>SNAGGSSPITGLVYDQRMMLHHNMWDSHHPELPQRISRIFSRHEELRLLSRCHRIPARLATEEELALCHSSKHISIIKSSEHMKPRDLNRLGDEYNSIFISNESYTCALLAAGSCFNSAQAILTGQVRNAVAIVRPPGHHAEKDTACGFCFFNTAALTARYAQSITRESLRVLIVDWDVHHGNGTQHIFEEDDSVLYISLHRYEDGAFFPNSEDANYDKVGLGKGRGYNVNIPWNGGKMGDPEYMAAFHHLVMPIAREFAPELVLVSAGFDAARGDPLGGFQVTPEGYAH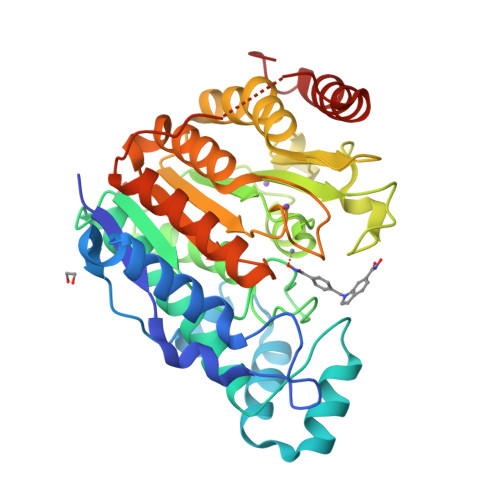LTHQLMSLAAGRVLIILEGGYNLTSISESMSMCTSMLLGDSPPSLDHLTPLKTSATVSINNVLRAHAPFWSSLR[2x]>[2x]MKILFVAAGSPATVFALAPLATAARNAGHDVFMGAVEDMVPYIASAGIPAVATTDLPIRHFITM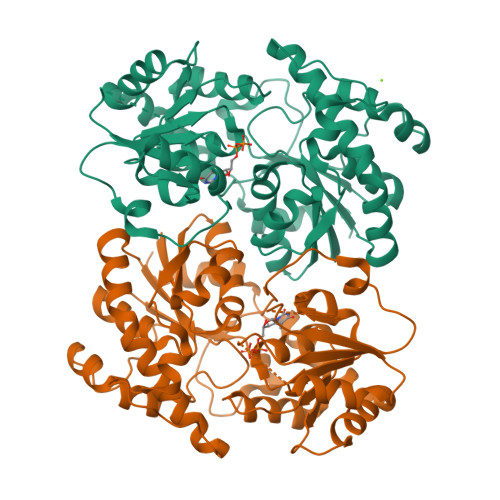DREGNPVRMPETPEEELDFAGHWFGRMAAGSMDALREVTANWRPDLVVGGSMSFAAALIAAELGVPYVRQAWDTGDAWRTDPAASDELRPELRALGLDRLPDPALFVDICPPSLRPADAPPAQMMRWVPANGQRRLEPWMYTKGNRPRILVTSGSRLVFAKKTGFLRGLVADMAALDAEVVIATLDEVAEELRTELPGVRAGWVPLDVVVPTCDVVVHHAGGVTALTAMNAGVPQLIVPQGGNFVEAGLRISDFGAAITVDENTPEAVEKACGELIGNPSYAERARELSAEIAALPLPAEVVGALEGLVENLYFQ> SQYEEKVRPCIDLIDSLRALGVEQDLALPAIAVIGDQSSGKSSVLEALSGVALPRGSGIVTRCPLVLKLKKLVNEDKWRGKVSYQDYEIEISDASEVEKEINKAQNAIAGEGMGISHELITLEISSRDVPDLTLIDLPGITRVAVGNQPADIGYKIKTLIKKYIQRQETISLVVVPSNVDIATTEALSMAQEVDPEGDRTIGILTKPDLVDKGTEDKVVDVVRNLVFHLKKGYMIVKCRGQQEIQDQLSLSEALQR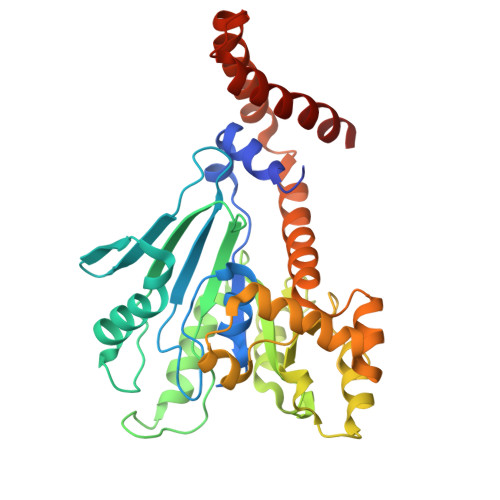EKIFFENHPYFRDLLEEGKATVPSLAEKLTSELITHISKSLPLLENQIKETHQRITEELQKYGGDPKAKFLKERLARLTQARRRLAQFPG The membrane protein FlhB is a highly conserved component of the flagellar secretion system. It is composed of an N-­terminal transmembrane domain and a C-terminal cytoplasmic domain (FlhBC). Flagellar FlhBC consists of a globular domain composed of a four-stranded β-sheet surrounded by four α-helices. The globular domain is preceded by a long N-terminal α-helix (α1) that connects the cytoplasmic globular part of FlhB to the transmembrane domain.

In the case of the AquFlhBC crystal there are three protein molecules in the asymmetric unit. The three molecules in the asymmetric unit are very similar, with r.m.s.d.s on pairwise superposition in the range 0.40–0.76 Å. Each molecule consists of two polypeptide chains resulting from proteolytic cleavage after Asn263. In all molecules no electron density was observed for residues 213–231 at the N-terminus; depending on the molecule, two to six residues at the C-terminus were disordered. In the SalFlhBC crystal α1 primarily contacts α1 and α2 of adjacent molecules, while in the AquFlhBC crystal α1 primarily contacts α4 and the cleavage site between β1 and β2. The major difference between SalFlhBC and AquFlhBC is in the N-­terminal region. However, a longer helix with a kink is not excluded in AquFlhBC, in which a highly conserved Gly230 occurs just two residues into the disordered segment 213–231 which is present in the crystallized protein but is absent in the model. A similar positive cleft is also present in AquFlhBC. Such a cleft might be a potential recognition site for proteins secreted by the flagellar secretion system.

>[3x]MKIMMSRRELKEEYKQLEGHPEVKSRIKARMRELAKSRMMAEVPKATVVITN;>PTHIAIALKYNPEKDKAPVVVAKGKGTIAQKIVEIAENYSIPVVRKPELARALYPAVEVGKEISPKFYKAVAEIIAYVMFKKKKVYA[3x]>[3x]MEKSNETNGYLDSAQAGPAAGPGAPGTAAGRARRCAGFLRRQALVLLTVSGVLAGAGLGAALRGLSLSRTQVTYLAFPGEMLLRMLRMIILPLVVCSLVSGAASLDASCLGRLGGIAVAYFGLTTLSASALAVALAFIIKPGSGAQTLQSSDLGLEDSGPPPVPKETVDSFLDLARNLFPSNLVVAAFRTYATDYKVVTQNSSSGNVTHEKIPIGTEIEGMNILGLVLFALVLGVALKKLGSEGEDLIRFFNSLNEATMVLVSWIMWYVPVGIMFLVGSKIVEMKDIIVLVTSLGKYIFASILGHVIHGGIVLPLIYFVFTRKNPFRFLLGLLAPFATAFATCSSSATLPSMMKCIEENNGVDKRISRFILPIGATVNMDGAAIFQCVAAVFIAQLNNVELNAGQIFTILVTATASSVGAAGVPAGGVLTIAIILEAIGLPTHDLPLILAVDWIVDRTTTVVNVEG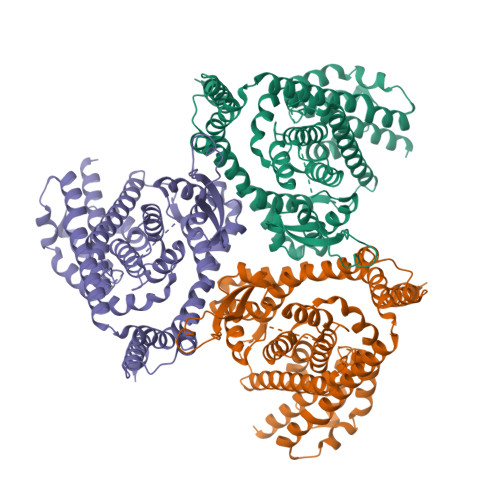DALGAGILHHLNQKATKKGEQELAEVKVEAIPNCKSEEETSPLVTHQNPAGPVASAPELESKESVL>[2x]HMSELSVATGAVSTASSSIPMPAGVNPADLAAELAAVVTESVDEDYLLYECDGQWVLAAGVQAMVELDSDELRVIRDGVTRRQQWSGRPGAALGEAVDRLLLETDQAFGWVAFEFGVHRYGLQQRLAPHTPLARVFSPRTRIMVSEKEIRLFDAGIRHREAIDRLLATGVREVPQSRSVDVSDDPSGFRRRVAVAVDEIAAGRYHKVILSRCVEVPFAIDFPLTYRLGRRHNTPVRSFLLQLGGIRALGYSPELVTAVRADGVVITEPLAGTRALGRGPAIDRLARDDLESNSKEIVEHAISVRSSLEEITDIAEPGSAAVIDFMTVRERGSVQHLGSTIRARLDPSSDRMAALEALFPAVTASGIPKAAGVEAIFRLDECPRGLYSGAVVMLSADGGLDAALTLRAAYQVGGRTWLRAGAGIIEESEPEREFEETCEKLSTLTPYLVARQ

MbtI from Mycobacterium tuberculosis (Mtb) is a Mg2+-dependent salicylate synthase, belonging to the chorismate-utilizing enzyme (CUE) family. MbtI converts chorismate to salicylate via a two-step mechanism, with the release of pyruvate. As a fundamental player in iron acquisition, MbtI promotes the survival and pathogenicity of Mtb in the infected host. MbtI is known to exist in two possible conformations, generally referred to as “open” and “closed”, depending on the position of two flexible loops relative to the active site, as extensively analyzed in our previous work.

In the context of our efforts to elucidate the binding mode of 5-phenylfuran-2-carboxylic acids to MbtI, we obtained co-crystals with 5-(3-carboxyphenyl)furan-2-carboxylic acid (II). Despite its modest inhibitory activity in vitro (IC50: 35.2 ± 2.6 μM; residual activity at 100 μM: 27.2% ± 4.5), the compound was chosen as part of a large panel of crystallization trials. In the case of MbtI-II, loop stabilization may have contributed to improve the overall resolution of the crystallographic data (up to 1.6 Å), leading to a significantly higher value than the one obtained for the MbtI-I dataset. Moreover, the electron density map for the active site region was clearly interpretable in all its parts, effectively providing a complete picture of the active site region around the ligand. In agreement with this hypothesis, the analysis of the ligand pose revealed the presence of an H-bond between the carboxylic group at position 3 of the phenyl and the main chain amide of Gly270. The binding mode of the compound was equivalent in the two MbtI protomers. The carboxylic moiety of the furan established H-bonds with the side chains of Tyr385, Arg405, and with the main chain amide of Gly419. The furan oxygen interacted with the guanidine group of Arg405. Finally, the carboxylic substituent on the phenyl ring formed H-bonds with Gly270 (as previously mentioned) and two ordered water molecules; one of them established a further interaction with the hydroxyl group of Thr271, while the other did so with the amine of Lys205. In our previous work, we speculated that the superior activity of I could be due to its ability to strongly bind this amino acid through its cyano group. This hypothesis is consistent with the present structure, which suggests a weaker interaction between compound II and MbtI Lys205, as evinced by the presence of an H-bond interaction between the ligand carboxylic group and the lysine ε-amino group, but a higher C-N distance (~3.20 Å) than that observed in the MbtI-I complex (2.29–2.82 Å over the four chains of the ASU).>GMVLTLSDLEKGYDKNLNQLSLSFLNLRDNDIPLLCEFLQNHPAITSLDLSHNDITANGVKLFVNKTSVSSLNISHNNIGPEGAQWLSEDNHITTLDVSFNEIGDEGVKALAANAKLITLYALYNKITKVGAGYLAQSNLKKIDLCFNSLEDEGVIALASNINIKELIASACDVSDIGAIELAKNNQLTLLILGKNAITDKSTLHFANNTSLSTLHLGSNQITAAGKKILETNTRITDLDLIGNPIEVHETDELNYSKKSPDSHSVFKFLQKFTFLSCMSPCQETAESDKGLNKKPN[8x];>[8x]GMAIAPQQIQERLKQEQYQKFVVADIGNFPHCLAQTPEGIASGQRYQKYSTNSLSRTPPFSQWGAPQLLTPKSAQEYIKFAQQRNKKSSFKIDGEAVRVSECSNFAYHSAGVLLDDPQIRTQYDVAVIGSMHSNGRYLHNITLLVPKGSRLPQPPQQLTAEVFPIGTLIVDPWAV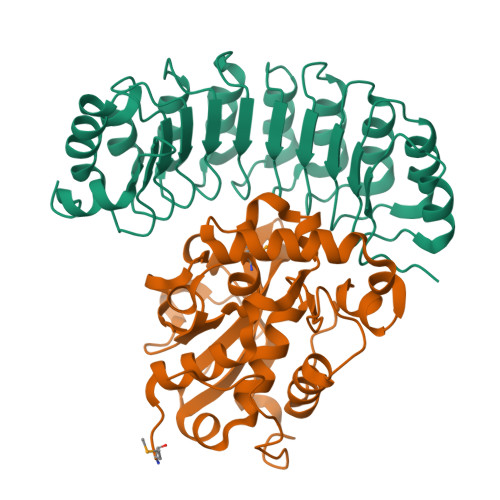GMGHPPEQALAIPKEQFAYNRSLFPATVNYQSALDESLTSTRTGQLTPYTGTPSRT>[2x]MIKGINHITYSVSNI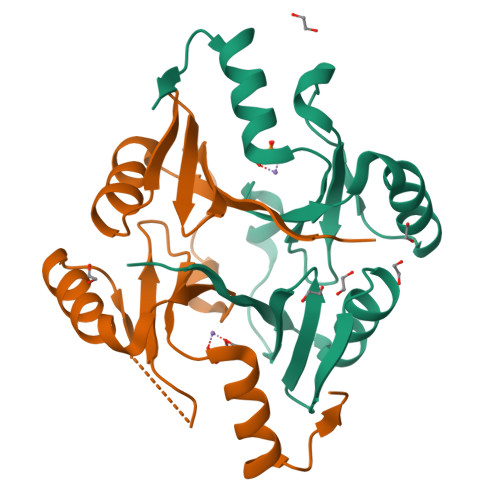AKSIEFYRDILGADILVESETLAYFNLGGIWLALNEEKNIPRSEIKYSYTHIAFTISDNDFEDWYNWLKENEVNILEGRDRDIRDKKSIYFTDLDGHKLELHTGSLEDRLSYYKEAKPHMNFYI> MHHHHHHASGLVPRGSRAWVSRGAHKLVGALEAFAIAVAGRRCLDAG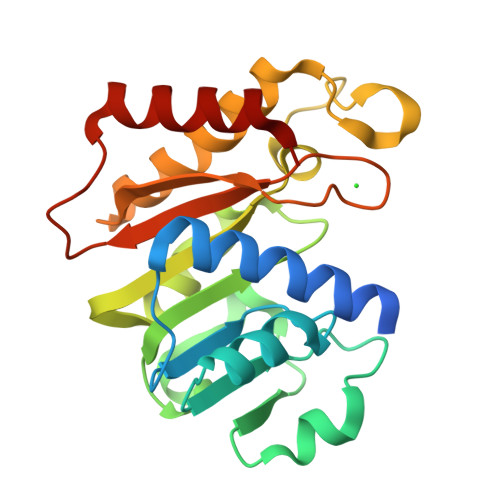ASTGGFTEVLLDRGAAHVVAADVGYGQLAWSLRNDPRVVVLERTNARGLTPEAIGGRVDLVVADLSFISLATVLPALVGCASRDADIVPLVKPQFEVGKGQVGPGGVVHDPQLRARSVLAVARRAQELGWHSVGVKASPLPGPSGNVEYFLWLRTQTDRALSAKGLEDAVHRAISEGP> GSHMASMKKKGSVVIVGRINLSGDTAYAQQTRGEEGCQETSQTGRDKNQVEGEVQIVSTATQTFLATSINGVLWTVYHGAGTRTIASPKGPVTQMYTNVDKDLVGWQAPQGSRSLTPCTCGSSDLYLVTRHADVIPVRRRGDSRGSLLSPRPISYLKGSSGGPLLCPAGHAVGIFRAAVSTRGVAKAVAFIPVESLETTMRSP

The HCV NS3/4A protease – a chymotrypsin-like serine protease – is a prime therapeutic target that cleaves four known sites along the virally encoded polyprotein. The NS3/4A protease also hydrolyzes two human proteins, TRIF and MAVS, which are part of the innate immune system, thereby confounding the innate immune response to viral infection. In this study, we report that four chemically representative protease inhibitors – telaprevir, danoprevir, vaniprevir and MK-5172 – exhibit distinct susceptibilities to the protease variants R155K, A156T and D168A. To elucidate the underlying mechanism by which chemically diverse inhibitors bind to the wild-type protease and drug-resistant variants, crystal structures were determined for 16 inhibitor-protease complexes. These complexes include wild-type protease and resistant variants R155K, D168A and A156T each bound to telaprevir, danoprevir, vaniprevir and MK-5172, with resolutions ranging from 1.10–2.50 Å; S139A protease variants were used except for telaprevir, which requires covalent bond formation with the serine 139 for efficient binding.

Telaprevir potency was slightly better against D168A relative to the wild type, while danoprevir, vaniprevir and MK-5172 lost 100- to 1000-fold potency against D168A. Interestingly, telaprevir showed better potency against the D168A variant than the wild-type; the crystal structure revealed that the P2 moiety bent considerably and packed closer against the D168A variant. The inhibitor shifted by approximately 0.5 Å relative the position in the wild-type complex, resulting in increased interactions with both R155 and A156. Telaprevir has reduced potency against R155K due to loss of van der Waals contacts but exhibits better potency against D168A as it allows tighter packing in the S2 subsite. Thus, while telaprevir's flexibility allows adaptation to D168A, it cannot accommodate the disruption by R155K or A156T. Telaprevir and other linear ketoamide drugs select for A156T variants by direct steric clashes, while linear (BI 201335) and macrocyclic drugs (danoprevir, vaniprevir, TMC435) with large P2 moieties select for D168A variants by disrupting favorable stacking interactions with R155. These data also support the converse observation that D168A variants are uncommon in patients treated with telaprevir as the drug can pack tighter in the S2 subsite.>[4x]MAHTGRMFKIEAAEIVVARLPLKFRFETSFGVQTHKVVPLLILHGEGVQGVAEGTMEARPMYREETIAGALDLLRGTFLPAILGQTFANPEAVSDALGSYRGNRMARAMVEMAAWDLWARTLGVPLGTLLGGHKEQVEVGVSLGIQADCQATVDLVRR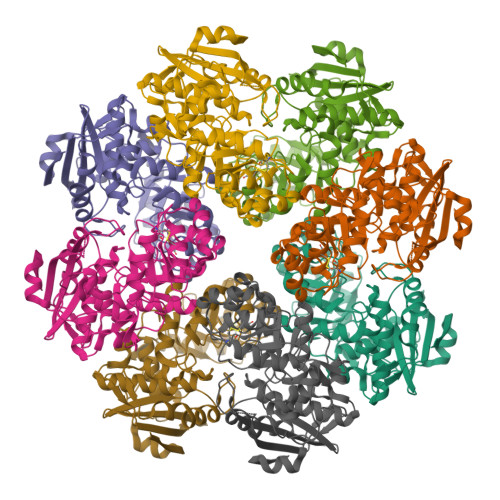HVEQGYRRIKLKIKPGWDVQPVRCTREAFPDIRLTVDANSAYTLADAGRLRQLDEYDLTYIEQPLAWDDLVDHAELARRIRTPLCLDESVASASDARKALALGAGGVINLKVARVGGHAESRRVHDVAQSFGAPVWCGGMLESGIGRAHNIHLSTLSNFRLPGDTSSASRYWERDLIQEPLEAVDGLMPVPQGPGTGVTLDREFLATVTEAQEEHRA> GAGCAGACAAG;> ACTGCACTCA;> C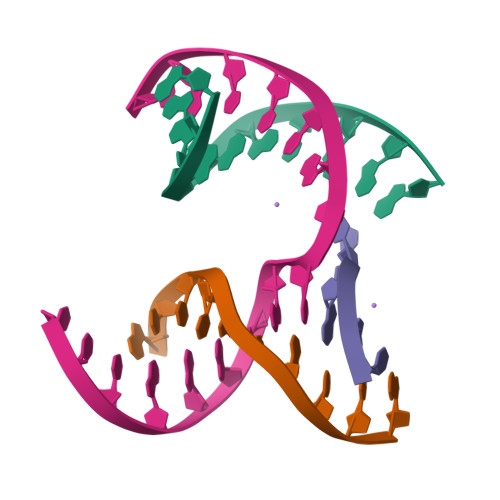TAGT;> TCTGAGTGCTGTCTGC>MTLSIPPSIQCQTEAACRLITRVTGDTLRAIHLYGSAVAGGLKPNSDIDLLVTICQPLTEAQRATLMQELLALSSPPGASAEKRALEVTVVLYSQLVPWCFPPSREMQFGEWLREDICQGIYEPAQQDWDMVLLITQILETSI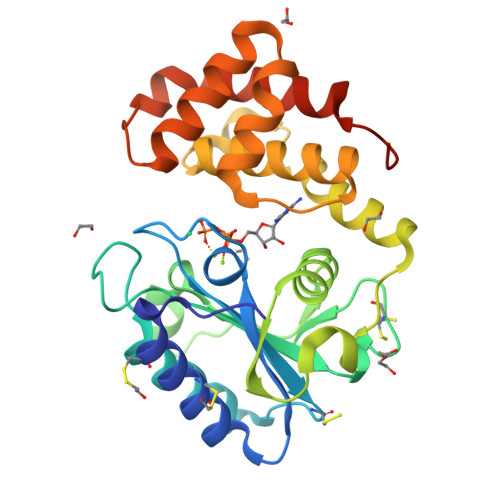PLKGERAERLFTPAPAAQLLKALRYPLDLWQSTADVQGDEYHIVLTLARIWYTLSTGRFTSKDAAADWLLPQLPEDYAATLRAAQREYLGLEQQDWHILLPAVVRFVDFAKAHIPTQFTKGHHHHHH[2x]> GKITFYEDRGFQGRHYECSSDHSNLQPYFSRCNSIRVDSGCWMIYEQPNFQGPQYFLRRGDYPDYQQWMGLNDSIRSCRLIPHTSSHRLRIYEREDYRGQMVEITEDCSSLHERFHFSEIHSFHVLEGWWVLYEMPNYRGRQYLLRPGDYRRYHEWG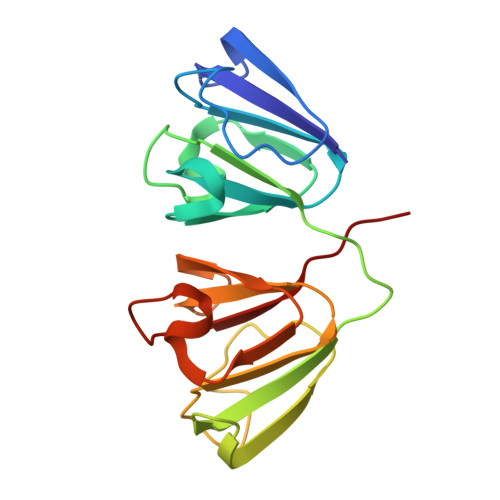AVDARVGSLRRAVDFY ethyl (2Z,4S)-4-{[(2R,5S)-5-amino-2-(4-fluorobenzyl)-6-methyl-4-oxoheptanoyl]amino}-5-[(3S)-2-oxopyrrolidin-3-yl]pent-2-enoate | C26 H36 F N3 O5 | 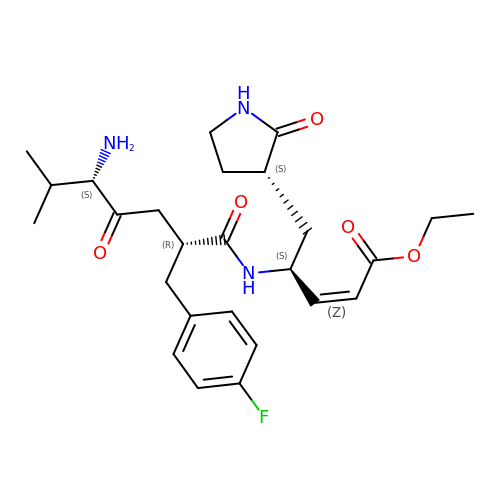XNNMMJDBDBVGGO-HSJYVMOXSA-N(3~{S},7~{S},8~{S})-7-oxidanyl-8-(phenylmethyl)-3-(pyridin-3-ylmethyl)-1,4,9-triazacyclotricosane-2,5,10-trione | C33 H48 N4 O4 | 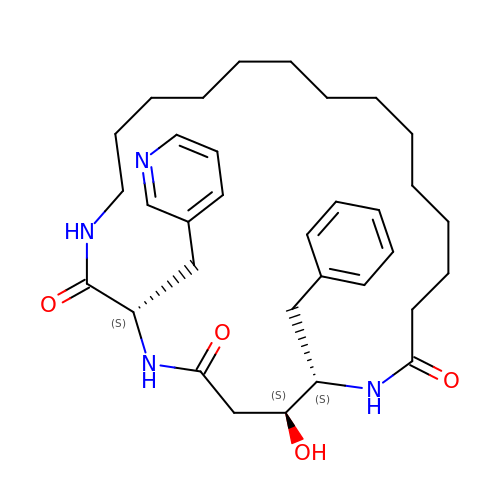RYGGELGJKGMCRW-DTXPUJKBSA-N>GSKDTDKDGIPDNKDACPEVPGLKEFNGCPDTDGDGIPDKDDACPQVKGPKEFNGCPDTDGDGIPDKDDACPEVAGPKEFNGCPDTDGDGIPDKDDKCPDVAGPAENGGCPWPDTDGDGVLDKDDLCPEVAGPASNKGCPEPDEKEQKQLNQYAKTILFDTGKATIKFQSAEVLNQIINVLKKYPNSRFRIEGHTDSTGKKAKNMILSQNRADAVKVYLIQGGIDAGRLESQGFGPEKPIASNKNKKGRELNRRVEINLIK[4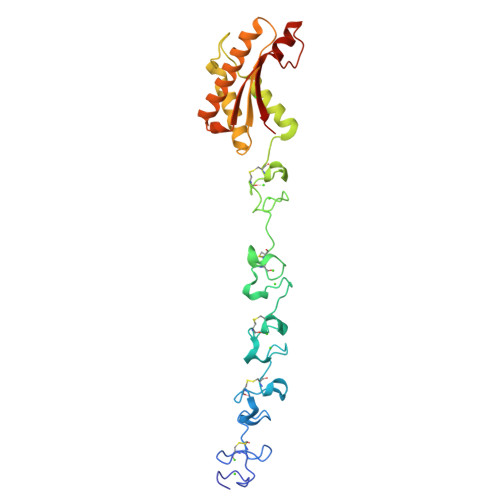x]>[3x]NGGVGVDVELITSINVENDTFIERNFTPQEIEYCSAQPSVQSSFAGTWSAKEAVFKSLGVKSLGGGAALKDIEIVRVNKNAPAVELHGNAKKAAEEAGVTDVKVS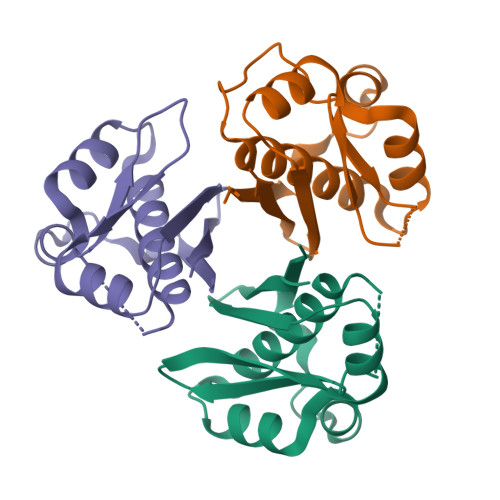ISHDDLQAVAVAVSTKK;>[3x]NGGVGVDVELITSINVENDTFIERNFTPQEIEYCSAQPSVQSSFAGTWSAKEAVFKSLGVKSLGGGAALKDIEIVRTNKNAPAVELHGNAKKAAEEAGVTDVKVSISHDDLQAVAVAVSTKK> QGAVRKATAAEIAALPRQKVELVDPPFVHAHSQVAEGGPKVVEFTMVIEEKKIVIDDAGTEVHAMAFNGTVPGPLMVVHQDDYLELTLINPETNTLMHNIDFHAATGALGGGGLTEINPGEKTILRFKATKPGVFVYHCAPPGMVPWHVVSGENGAIMVLPREGLHDGKGKALTYDKIYYVGEQDFYVPRDENGKYKKYEAPGDAYEDTVKVMRTLTPTHVVFNGAVG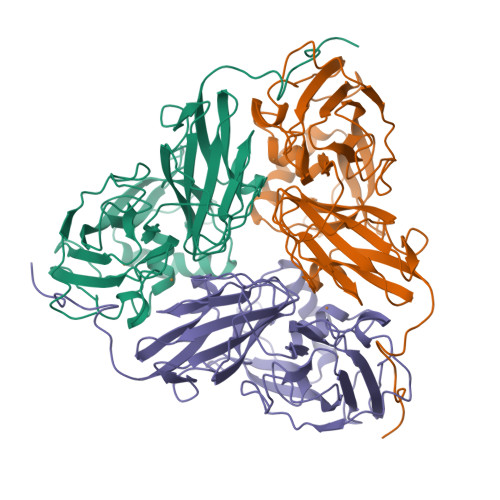ALTGDKAMTAAVGEKVLIVHSQANRDTRPHLIGGHGDYVWATGKFNTPPDVDQETWFIPGGAAGAAFYTFQQPGIYAYVNHNLIEAFELGAAAHFKVTGEWNDDLMTSVLAPSGT> MIHYFDYSMMRIPLIFPLCMVALLSG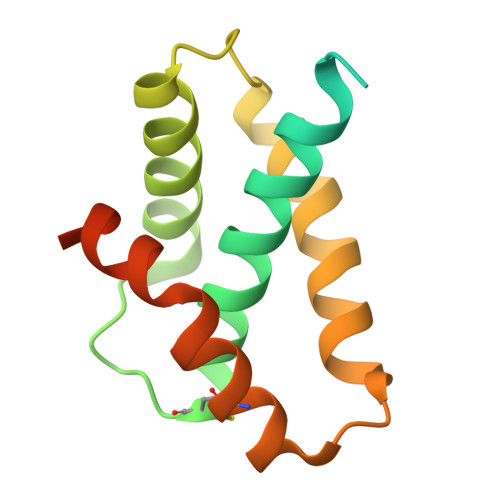CQQKPASTLSPAISSQAQLEQLSSVAAGTRYLKNKCNRSDLPADETIYRAAVNVGKARGWGNIDVATLSQNSDRLYQQLLQDSTPEATQCSQFNRQLAPFIASLRSDGSDYKDDDDK>TTVTIVRKDGRIAIAADTLTKWGGGKESADYVANHEKIIRVGDSYVAITGSATFKLILADYFASLDEPPQLDSVARIFCVWNTLHGALKEHYYLQAGEDKEDDLESSRMDVLIANPRGIFGVAAHRTVQEFSKFYAYGSGSPYALGAMYAAYRAPSLDAEAVARLGVMAAAEFHDESGLPVQSFVMELSPDVGS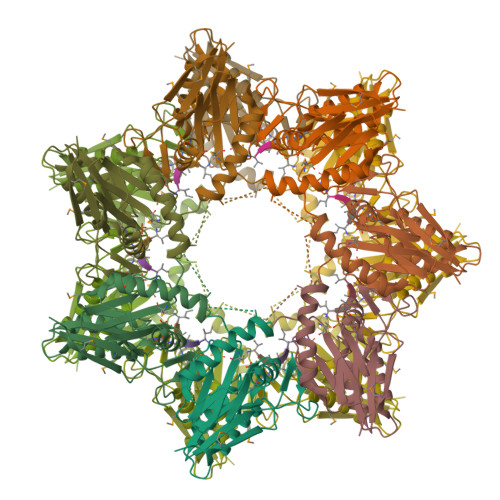GENLYFQ[7x]> MEALIPVINKLQDVFNTVGADIIQLPQIVVVGTQSSGKSSVLESLVGRDLLPRGTGIVTRRPLILQLVHVSQEDKRKTTGEENGVEAEEWGKFLHTKNKLYTDFDEIRQEIENETERISGNNKGVSPEPIHLKIFSPNVVNLTLVDLPGMTKVPVGDQPKDIELQIRELILRFISNPNSIILAVTAANTDMATSEALKISREVDPDGRRTLAVITKLDLMDAGTDAMDVLMGRVIPVKLGIIGVVNRSQLDINNKKSVTDSIRDEYAFLQKKYPSLANRNGTKYLARTLNRLLMHHIRDCLPELKTRINVLAAQYQSLLNSYGEPVDGSGSGSGSKEAADMLKALQGASQIIAEIRETHLWLEHHHHHH

DNM1L is targeted from the cytoplasm to the outer mitochondrial membrane (MOM) and is a key player in mitochondrial fission. Similar to previous studies for human dynamin and Arabidopsis thaliana A (AtDrp1A), we designed a fusion protein comprising the GTPase domain (G) and the bundle signaling element (BSE, B) of human DNM1L (the so-called GTPase domain - GED (GG) construct). The stalk (S), which participates in higher-order oligomerization, and the B-insert were replaced by a GSGSGSGS linker, which continued with the C-terminal helix of the BSE. The GTPase domain of human DNM1L consists of a central eight-stranded β-sheet surrounded by seven α-helices and two one-turn helices resembling the GTPase core of mammalian dynamin-1.

In the nucleotide-free form, a citrate from the crystallization buffer is bound to the P-loop, mimicking the phosphate moiety of GTP. Apparently, the citrate compensates charges in the active site of DNM1L, while the GMP-PNP occupied active site exhibits a distinct conformation in the P-loop and switch I. In GMP-PNP-DNM1L, the side chain of Arg53 extends to the bulk solvent above the GTP-binding groove, whereas in the nucleotide-free form, this side chain is hydrogen-bonded to Ser40 and Glu43, in a position similar to that of the nucleotide-loaded dynamin complex. This translocation in the nucleotide-free state may be an artificial charge compensation for the negative charge of the P-loop bound citrate. Interestingly, the water molecule in our nucleotide-free DNM1L GG construct is in the same position as the catalytic water in dynamin-1. This catalytic water connects switch I with switch II via hydrogen bonds to the Thr59 carbonyl oxygen and the Gly149 NH, respectively. The overall root mean square deviation (RMSD) between the nucleotide-free and –bound DNM1L GG construct is only 0.69 Å for the Cα atoms, indicating almost identical structures. The BSE is formed by the N-terminal helices α1B (residues 4–16) and α1AB, helix α2B (303–323) and the C-terminal helix α3B (708–729, with residues S708GS710 from the artificial linker), arranged in a three-helix bundle with an additional one-turn helix. Both our structures represent the closed conformation of the BSE in relation to the GTPase domain, which has been called the “post-fission state”.Pseudomonas aeruginosa CtpA is a carboxyl-terminal processing protease that partners with the outer membrane lipoprotein LbcA to degrade at least five cell wall-associated proteins, four of which are cell wall hydrolases. Instead, it requires the adaptor protein LbcA, the lipoprotein-binding partner of CtpA, for activity in vivo and in vitro. Therefore, it appears that LbcA interacts with CtpA to assemble an active proteolytic complex, which controls the activity of these enzymes by degrading them. We show that CtpA alone assembles as an inactive trimer of dimers and that LbcA is a right-handed spiral that might wrap around a substrate protein.

We then produced selenomethionine-substituted CtpA crystals for single-wavelength anomalous diffraction (SAD)-based phasing. The derivatized crystals diffracted to 3.3 Å, leading to successful structural solution. There are two CtpA molecules in one asymmetric unit (ASU), and CtpA formed a hexamer that comprised a trimer of dimers in crystal. As expected, each CtpA protomer consists of an N-terminal dimerization region (NDR), a PDZ domain, a cap domain, a protease core domain, and a C-terminal dimerization region (CDR). The PDZ domain is partially disordered, but we generated a homolog PDZ model based on the CtpB structure and accurately docked the domain guided by two anomalous density peaks from selenomethionine residues 153 and 160 of the domain. The CtpA catalytic Ser-302 is located at the end of the narrow tunnel between the cap and the body region. The PDZ domain is in a position that blocks the narrow substrate peptide tunnel leading to Ser-302. Furthermore, the catalytic triad Ser-302–Lys-327–Gln-331 is well beyond hydrogen-bonding distance: Ser-302 and Lys-327 are 4.2 Å apart, and Lys-327 and Gln-331 are 9.1 Å apart. By superimposing the two proteases, we found that transition to the active form requires the CtpA cap domain to clamp down toward the catalytic site by 11 Å and also a large-scale movement of the associated PDZ domain by 12 Å. However, the six unhinged CDRs of three CtpA dimers interact to form the triangular trimer-of-dimer complex.

>GSHMSAPLPLDELRTFAEVLDRVKAAYVEPVDDKTLLENAIKGMLSNLDPHSAYLGPEDFAELQESTSGEFGGLGIEVGSEDGFIKVVSPIDDTPAARAGIQPGDLIVQIDGKPTKGQSMTEAVDSMRGKAGSPITLTIVRDGGRPFDVELKRAIIKVKSVKSQVLEPGYAYLRITQFQVNTGEEVVKALNQLRKDNKGRLKGLVLDLRNNPGGVLQSAVEVADAFLTKGLIVYTKGRIANSELRFSADPADPSDKVPLVVLINGGSASAAEIVAGALQDQKRAILMGTDSFGKGSVQTVLPLNNDRALKLTTALYYTPNGRSIQAQGIVPDIEVGRAKVTQERSSFEGFKEADLQGHLANGNGGADRPTGKRAAPSERPQDSDYQLSQALSLLKGLSVTRGN[2x]> FMVSLPRMVYPQPKVLTPCRKDVLVVTPWLAPIVWEGTFNIDILNEQFRLQNTTIGLTVFAIKKYVAFLKLFLETAEKHFMVGHRVHYYVFTDQPAAVPRVTLGTGRQLSVLEVRAYKRWQDVSMRRMEMISDFCERRFLSEVDYLVCVDVD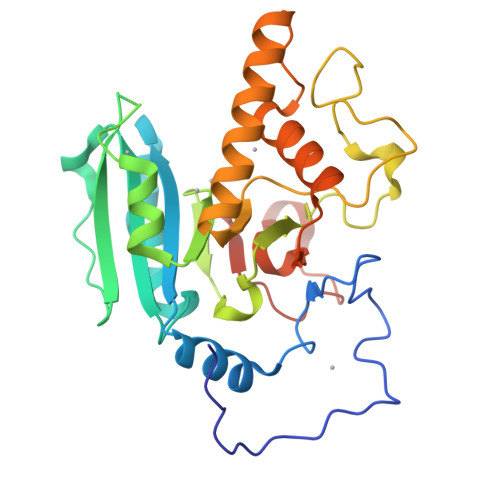MEFRDHVGVEILTPLFGTLHPGFYGSSREAFTYERRPQSQAYIPKDEGDFYYLGGFFGGSVQEVQRLTRACHQAMMVDQANGIEAVWHDQSHLNKYLLRHKPTKVLSPEYLWDQQLLGWPAVLRKLRFTAVPKNHQAVRNPE> GAMGRRPEEWGKLIYQWVSRSGQNN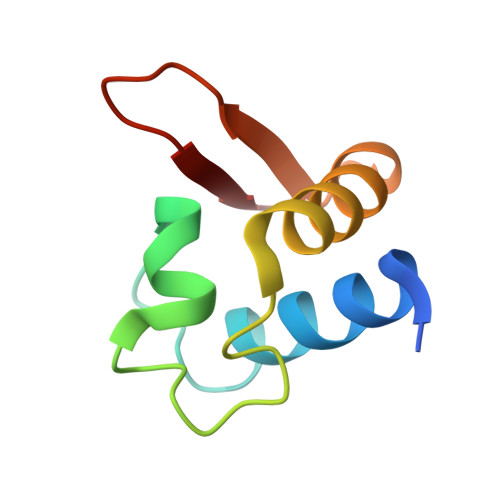SVFTLYELTNGEDTEDEEFHGLDEATLLRALQALQQEHKAEIITVSDGRGVKFF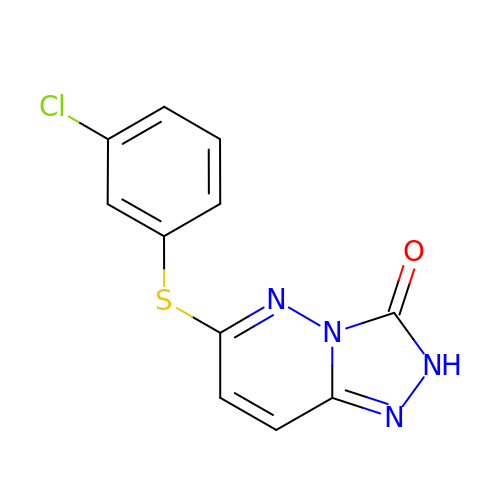3-(3-chlorophenyl)sulfanyl-1$l^{4},2,7,8-tetrazabicyclo[4.3.0]nona-1(6),2,4,7-tetraen-9-one | C11 H7 Cl N4 O S | ONDJIHGHEXNTAW-UHFFFAOYSA-N O-[(S)-({(2R)-2,3-bis[(9Z)-octadec-9-enoyloxy]propyl}oxy)(hydroxy)phosphoryl]-L-serine | C42 H78 N O10 P | 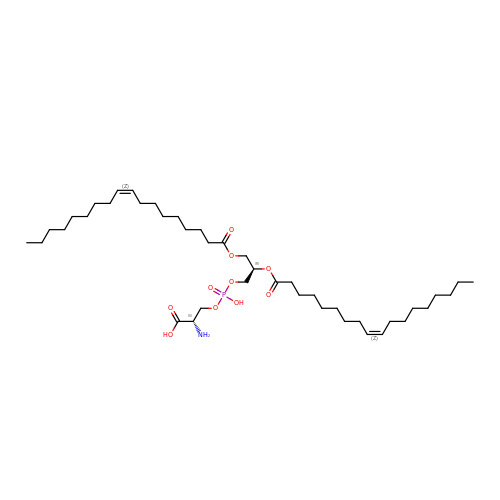WTBFLCSPLLEDEM-JIDRGYQWSA-N>[6x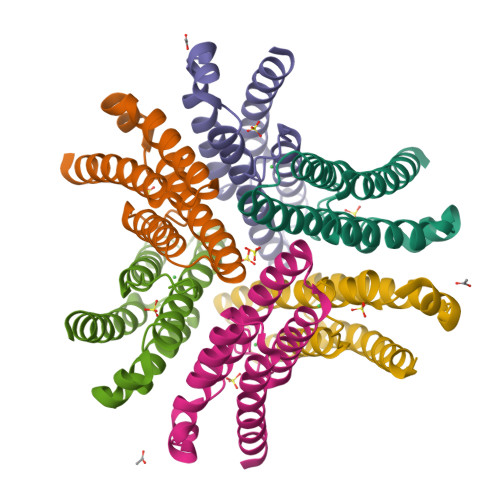]HCDLPCGVYDPAQARIEAESVKAIQEKMAANDDLHFQIRATVIKEQRAELAKHHLDVLWSDYFKPPHFESYPELHTLVNEAVKALSAAKASTDPATGQKALDYIAQIDKIFWETKKA DGC domains containing the signature GGDEF motif synthesise c-di-GMP from two GTP molecules while EAL1516 and HD-GYP171819 domain-containing PDEs are responsible for the hydrolysis of c-di-GMP to 5′-phosphoguanylyl-(3′-5′)-guanosine (pGpG). Hydrolysis of c-di-GMP by EAL domains has been shown to require the presence of divalent ions, either Mg2+ or Mn2+, with the most efficient reactions occurring at alkaline pH2933. Here we report as yet structurally uncharacterised EAL domains from the core genome of Pseudomonas aeruginosa, PA1727 (MucR) and PA3825.

We were fortuitous to observe PA3825EAL with bound product pGpG, from co-crystallisation with c-di-GMP and Mn2+. In this complex, the M1 site in the pGpG-bound structure is superimposable to the M1 metal in Mg2+ and Ca2+ complexes, the M2 site is vacant, but we observed a solvent binding site that interacts directly with the bound pGpG that presents metal like coordination geometry. We propose this as a potential third metal binding site, designated as M3. Diffraction data collected above the manganese absorption edge confirmed the presence of Mn2+ in the M1 position in the pGpG/Mn2+ PA3825EAL complex but showed no signal for manganese at the M3 metal like centre. Consistent with the absence of any anomalous signal in the M3 site, we have placed and refined sodium in this location which is abundant in the crystallisation condition and consistent with the geometry observed. The M3 metal site displays a tetrahedral coordination sphere consisting of Asp 160, a water molecule, the ribose O2′ oxygen and a P1 hydroxyl oxygen from pGpG. In PA3825EAL, the M2 site is empty, but Glu217 (contributed by the β7-α7 loop in close vicinity to the β5-α5 loop) replaces interactions with the phosphate moiety normally made by M2. While PA3825EAL lacks a metal in the M2 site and possesses one in the M3 site, the comparison with CC3396EAL, in which all three metal sites are occupied, suggests M3 site is a bona fide metal binding site in PA3825EAL. Instead, the M3 metal is observed in the product state where it is ideally poised to stabilise the negatively charged transition state during hydrolysis of c-di-GMP to pGpG; where pGpG directly contributes to formation of the M3 metal site via its non-bridging phosphate oxygen (terminal phosphate group of pGpG). The data presented also allows the identification of a third metal site M3 which is a hallmark of the product state.

> ASPSSELRRALEANEFIPYYQPLSPGQGGRWIGVEVLMRWRHPREGLIRPDLFIPFAERSGLIVPMTRALMRQVAEDLGGHAGKLEPGFHIGFNISATHCHELALVDDCRELLAAFPPGHITLVLELTERELIESSEVTDRLFDELHALGVKIAIDDFGTGHSSLAYLRKFQVDCLKIDQSFVARIGIDTLSGHILDSIVELSAKLDLDIVAEGVETPEQRDYLAARGVDYLQGYLIGRPMPLESLLSSLTVQE NA is a homotetrameric transmembrane glycoprotein responsible for cleavage of sialic acid from the host cell membrane. By blocking NA enzymatic activity, neuraminidase inhibitors (NAIs) prevent new viral particles from being released from the surface of an infected cell, thus stopping the spread of virus in the airways. In this study, we applied a set of experimental techniques using recombinant NA variants to understand the molecular basis of development of oseltamivir resistance in the viral N1 neuraminidase NA2009. To decipher the structural mechanism of resistance, we determined crystal structures of NA2009 mutants in complex with oseltamivir carboxylate.

Two variants (I223V and S247N single mutants) crystallized in the centered orthorhombic space group with two molecules in the asymmetric unit; the tetrameric biological unit could be reconstructed from two symmetrically related dimers. Residue 247 is located at the edge of the enzyme active site. As its side chain is exposed to the solvent, substitution of serine with the larger asparagine (S247N mutation) does not induce changes in the protein structure; the RMSD for superposition of 390 Cα with the wt structure was 0.133 Å. Nevertheless, changes in the structure of the hydration shell were observed. Namely, N247 is involved in a water-mediated contact with the oxygen atom in the pentyloxy substituent of oseltamivir, an interaction that is not present in the wt enzyme. S247 forms hydrogen bonds with two water molecules present only in the wt enzyme and not in the S247N mutant. The effects of the I223V and S247N single mutations were more modest (approximately 30- and 20-fold increases in Ki, respectively). The entropic contribution of oseltamivir binding to S247N NA2009 was almost unaffected; the value was within experimental error of the wt value. Rather, small structural alterations—such as loss of a dispersion bond with oseltamivir in the V223 mutant and changes in the hydration shell in the N247 mutant—appear responsible for increases in Ki.

>SVKLAGNSSLCPVSGWAIYSKDNSVRIGSKGDVFVIREPFISCSPLECRTFFLTQGALLNDKHSNGTIKDRSPYRTLMSCPIGEVPSPYNSRFESVAWSASACHDGINWLTIGISGPDNGAVAVLKYNGIITDTIKSWRNNILRTQESECACVNGSCFTVMTDGPNNGQASYKIFRIEKGKIVKSVEMNAPNYHYEECSCYPDSSEITCVCRDNWHGSNRPWVSFNQNLEYQIGYICSGIFGDNPRPNDKTGSCGPVSSNGANGVKGFSFKYGNGVWIGRTKSISSRNGFEMIWDPNGWTGTDNNFSIKQDIVGINEWSGYSGSFVQHPELTGLDCIRPCFWVELIRGRPKENTIWTSGSSISFCGVNSDTVGWSWPDGAELPFTIDK[2x]> AHMAPLSSDELKTVVSVLA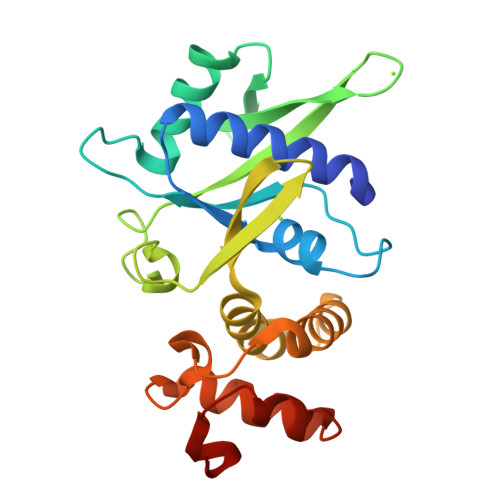QKLDSLNIDYAIMGGAATCLLSGDPNRRTEDVDLVIHVDHRKITADNLTTQLLKSFPSDFEGVSQFGHTIPAYKLRRPGGTVQLVELEVFDYQSWPQRPQYDLQTATRTTLNINGQKVKLFSPEWILREKILSQYQRQGSRKEGTDIRDIISMIPLAVPGKPELNFNQSQELQTALANLVQKRPDLSSALKAKIKCSAVFHN> MFNDRVIVKKSPLGGYGVFARKSFEKGELVEECLCIVRHNDDWGTALEDYLFSRKNMSAMALGFGAIFNHSKDPNARHELTAGLKRMRIFTIKPIAIGEEIT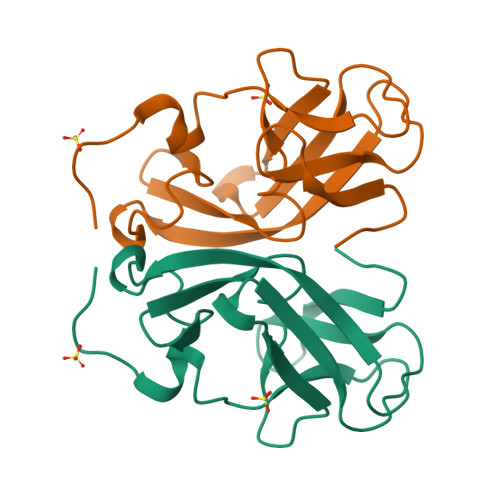ISYGDDYWLSRPRLTQN3-(3-fluorophenyl)benzoic acid | C13 H9 F 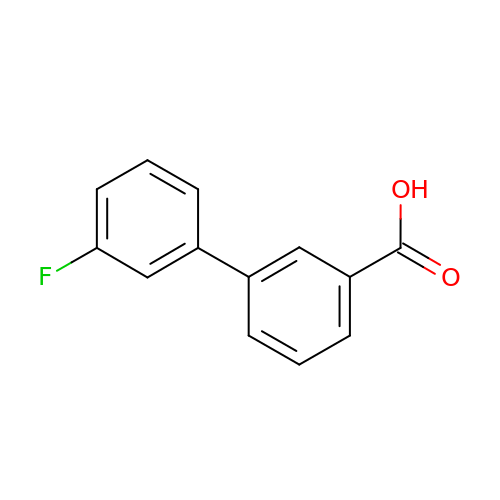O2 | MZZYPWIFSCZUHN-UHFFFAOYSA-N N-(5-amino-2,6-dioxo-1,2,3,6-tetrahydropyrimidin-4-yl)-5-O-phosphono-beta-D-ribofuranosylamine 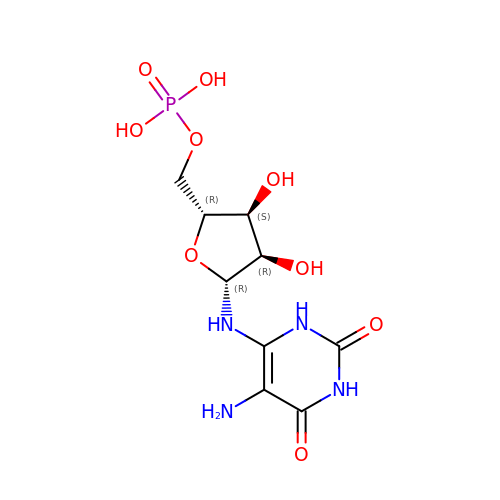| C9 H15 N4 O9 P | LZEXYCAGPMYXLX-UMMCILCDSA-N> ETFEIPESVTMSPKQFEGYTPKKGDVTFNHASHMDIACQQCHHTVPDTYTIESCMTEGCHD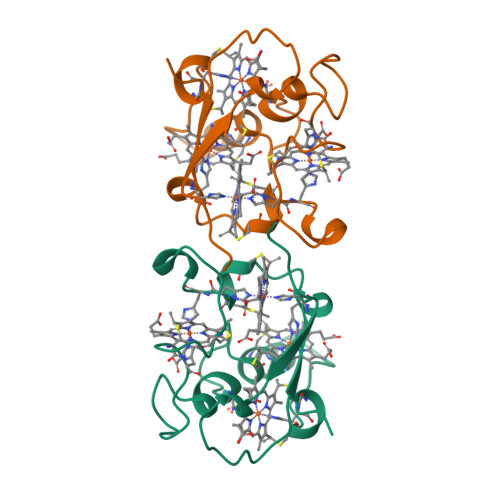NIKERTEISSVERTFHTTKDSEKSCVGCHRELKRQGPSDAPLACNSCHVQ>[2x]MHHHHHHE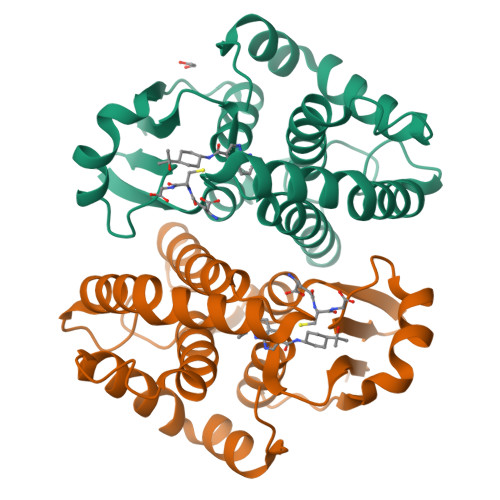NLYFQGMPNYKLTYFNMRGRAEIIRYIFAYLDIQYEDHRIEQADWPEIKSTLPFGKIPILEVDGLTLHQSLAIARYLTKNTDLAGNTEMEQCHVDAIVDTLDDFMSCFPWAEKKQDVKEQMFNELLTYNAPHLMQDLDTYLGGREWLIGNSVTWADFYWEICSTTLLVFKPDLLDNHPRLVTLRKKVQAIPAVANWIKRRPQTKL> GPLLEMILITGSNGQLGTELRYLLDERGVDYVAVDVAEMDITNEDKVEAVFAQVKPTLVYHCAAYTAVDAAEDEGKALNEAINVTGSENIAKACGKYGATLVYISTDYVFDGNKPVGQEWVETDHPDPKTEYGRTKRLGELAVERYAEHFYIIRTAWVFGNYGKNFVFTMEQLAENHSRLTVVNDQHGRPTWTRTLAEFMCYLTENQKAFGYYHLSNDAKEDTTWYDFAKEILKDKAVEVVPVDSSAFPAKAKRPLNSTMNLDKAKATGFVIPTWQEALKAFYQQGLKK

We show that gacA is an essential gene of GAS that encodes a metal‐independent dTDP‐4‐dehydrorhamnose reductase representative of a new class of monomeric RmlD enzymes. Bioinformatics analysis suggests that gacA encodes a dTDP‐4‐dehydrorhamnose reductase, an enzyme that catalyzes the final step in the production of dTDP‐L‐rhamnose. In general, RmlD enzymes are members of the large short‐chain dehydro‐genases/reductases (SDR) superfamily, which act on a wide family of substrates and commonly form homo‐dimeric or multimeric complexes (Kavanagh et al., 2008). GAS expresses a characteristic SCWP known as Lancefield Group A Antigen or Group A Carbohydrate (GAC).

To unravel why GacA functions as a monomer, we employed X‐ray crystallography. Crystals diffracted routinely below 1.2 Å and were subjected to synchrotron data collection. Consistent with our SEC and activity studies, GacA crystallized as a monomer. GacA contains the typical α‐helical/β‐sheet arrangement known as Rossmann fold present in SDR domains. In agreement with the well‐characterized SeRmlD (Blankenfeldt et al., 2002), the GacA β‐sheet is formed of six β‐strands, in the order 213457. This β‐sheet is flanked by three and four α‐helices on either side, respectively. The second 310‐helix η2 observed in SeRmlD (Blankenfeldt et al., 2002) is missing in GacA due to a shorter loop connecting α‐helix α7 and β‐strand β7. In comparison with SeRmlD, α8 from GacA lacks two α‐helical turns, due to a deletion of eight amino acids in GacA. No symmetry‐related GacA molecule forms protein–protein interactions via α1 and α10 as observed in SeRmlD (Blankenfeldt et al., 2002).> GSDPLKIADQSVDLNLKLMKWRILPDLNLDIIKNTKVLLLGAGTLGCYVSRALIAWGVRKITFVDNGTVSYSNPVRQALYNFEDCGKPKAELAAASLK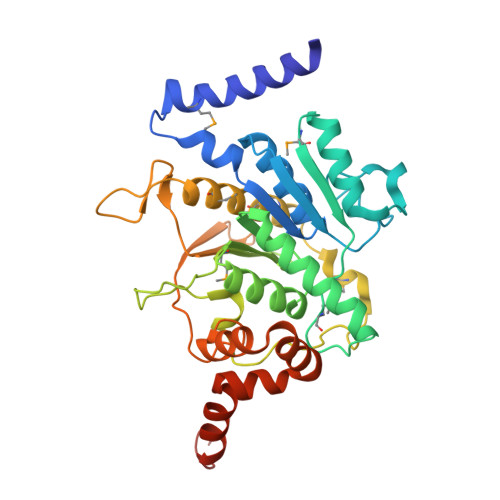RIFPLMDATGVKLSIPMIGHKLVNEEAQHKDFDRLRALIKEHDIIFLLVDSRESRWLPSLLSNIENKTVINAALGFDSYLVMRHGNRDEQSSKQLGCYFCHDVVAPTDSLTDRTLDQMSTVTRPGVAMMASSLAVELMTSLLQTKYSGSETTVLGDIPHQIRGFLHNFSILKLETPAYEHCPACSPKVIEAFTDLGWEFVKKALEHPLYLEEISGLSVIKQEVERLGNDVFEWEDDESDEIA> MVQELSIERLLEMESLVADPSEEFQFLRVGPDSNVPPKFRAPVSSLCQIGNKQIAALVVWARDIPHFSQLEMEDQILLIKGSWNELLLFAIAWRSMEFLTEERDGVDGTGNRTTSPPQLMCLMPGMTLHRNSALQAGVGQIFDRVLSELSLKMRTLRVDQAEYVALKAIILLNPDVKGLKNRQEVEVLREKMFLCLDEYCRRSRSSEEGRFAALLLRLPALRS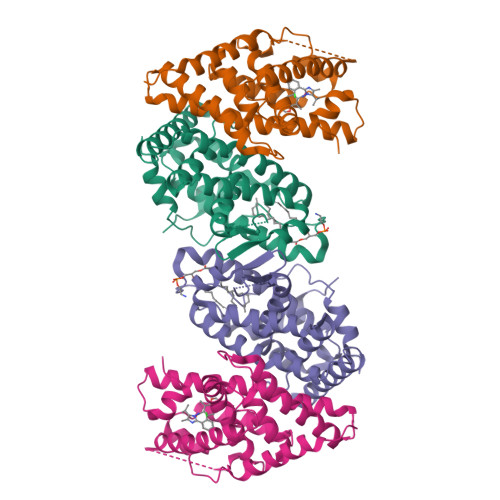ISLKSFEHLFFFHLVADTSIAGYIRDALRNHAPPIDTNMM;> GSHMASMTGGQQMGRDPKNVPPLTANQKSLIARLVYYQEGYEQPSEEDLKRVTQTWQSDEDDEDSDMPFRQITEMTILTVQLIVEFAKGLPGFSKISQSDQITLLKACSSEVMMLRVARRYDAATDSVLFANNQAYTRDNYRKAGMAYVIEDLLHFCRCMYSMMMDNVHYALLTAIVIFSDRPGLEQPSLVEEIQRYYLNTLRVYILNQNSASPRSAVIFGKILGILTEIRTLGMQNSNMCISLKLKNRKLPPFLEEIWDVADVA> SPSAEACGYSDRVLQLKLGNSAIVTQEAANYCCAYGEWPNYLPDHEAVAIDKPTQPETATDRFYTLRSVKWEATSTGWWWKLPDALNNIGMFGQNVQHHYLYRSGFLIHVQCNATKFHQGALLVVAIPEHQRGAHNTTTSPGFDDIMKGEAGGTFNHPYVLDDGTSLACATIFPH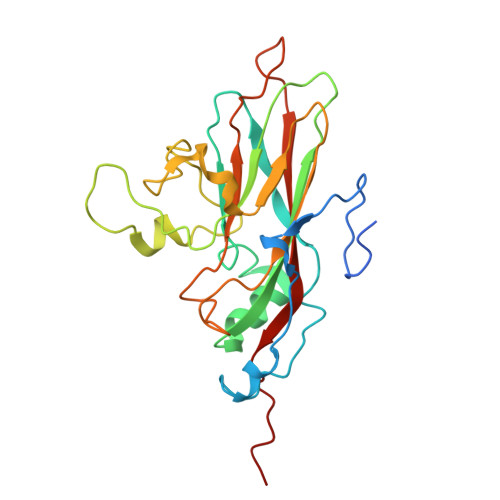QWINLRTNNSATIVLPWMNAAPMDFPLRHNQWTLAIIPVVPLGTRTMSSMVPITVSIAPMCCEFNGLRHAITQ>[4x]MAHHHHHHMKALYTTIAKAHGGRNGHVETTDGLLKLDLAMPRELGGEGGATNPEQLFAAGYAACFESAIRHVANVQKISLEDVSMTSEVSLYATPEKGFKLGVALHAH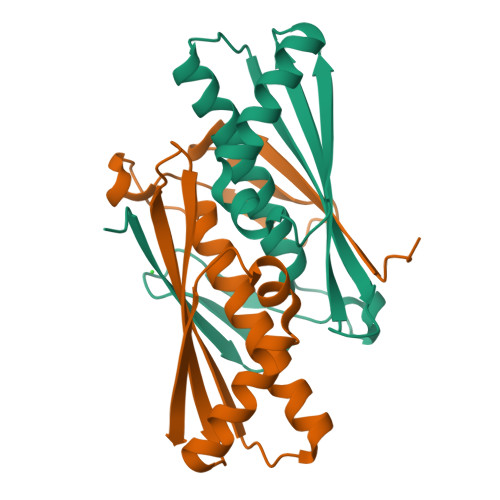ITGLNQNEAEALVAKAHEVCPYSNAIRGNVDVKLSVSVK>PMAAHEASSLYSEEKAKLLREMMAKIEDKNEVLDQFMDSMQLDPETVDNLDAYSHIPPQLMEKCAALSVRPDTVRNLVQSMQVLSGVFTDVEASLKDIRDLLEEDELLEQKFQEAVGQAGAISITSKAELAEVRREWAKYMEVHEKASFTNSELHRAMNLHVGNLRLLSGPLDQVRAALPTPALSPEDKAVLQNLKRILAKVQEMRDQRVSLEQQLRELIQKDDITASLVTTDHSEMKKLFEEQLKKYDQLKVYLEQNLAAQDRVLCALTEANVQYAAVRRVLSDLDQKWNSTLQTLVASYEAYEDLMKKSQEGRDFYADLESKVAALLERTQSTCQAREAARQQLLDRELK[2x]

HD-PTP (His domain protein tyrosine phosphatase; PTPN23) is a non-receptor tumor suppressor phosphatase (Kok et al., 1997, Toyooka et al., 2000) that regulates several ubiquitin-dependent endosomal trafficking processes such as downregulation of EGFR and PDGFRβ signaling (Doyotte et al., 2008, Ma et al., 2015), recycling of Src (Chen et al., 2012, Lin et al., 2011), and degradation of α5β1 integrin (Kharitidi et al., 2015). HD-PTP drives the degradation of mitogenic receptors by coordinating their sorting into the multivesicular body (MVB) via specific recruitment of different endosomal sorting complexes required for transport (ESCRTs) (Ali et al., 2013, Stefani et al., 2011). HD-PTP has a multidomain organization that allows coordinated binding to several ESCRTs. The CC domain of HD-PTP is solely responsible for the interaction with UBAP1, and residue F678 in this domain is essential for binding (Stefani et al., 2011).

The crystallographic structure of HD-PTPCC (apo-HD-PTPCC), determined at 2.5 Å resolution, shows an elongated architecture with seven α helices (H1–H7) whose main feature is a central helix of 105 residues (H7) extending the whole length of the molecule. The overall shape resembles that of an ice hockey stick, in which H1, H6, and the N-terminal region of H7 form the blade, and H2–H5 and the rest of H7 form the shaft. The maximal dimension of HD-PTPCC is approximately 155 Å from end to end. Analysis of the structure using SOCKET identified two canonical coiled-coil motifs: one antiparallel two-stranded coil involving helices H6 and H7 in the blade and an extensive antiparallel, tightly packed three-stranded coil involving helices H3, H4, and H7 in the shaft. The topology of HD-PTPCC is such that the polypeptide chain crosses three times over the length of the protein. The extended shape of HD-PTPCC differs markedly from the V domains of Alix (AlixV) and yeast Bro1 (Bro1V) (Fisher et al., 2007, Lee et al., 2007, Pashkova et al., 2013). By contrast, in HD-PTPCC, helix H7 forms a continuous backbone that confers rigidity to the molecule. The DEER analysis is therefore consistent with an overall rigid conformation for HD-PTPCC that can accommodate local flexibility without global rearrangements, ruling out a potential mechanism of regulation by large-scale flexibility of the CC domain. Pocket A is partially occluded in the structure of apo-HD-PTPCC by the side chains of K671, D667, and E514. In the apo-HD-PTPCC structure, D667 and K671 form a salt bridge, and the carboxyl group of E514 is about 6.4–7 Å to D667 and K671.>MSGGSTDVAMLSWLAALPATLGQVKDLEITSFKYDGQRGEVRIHARSSDFQPFEQARVKLAEKFNVEQGQLNRSDNVVMGSFVL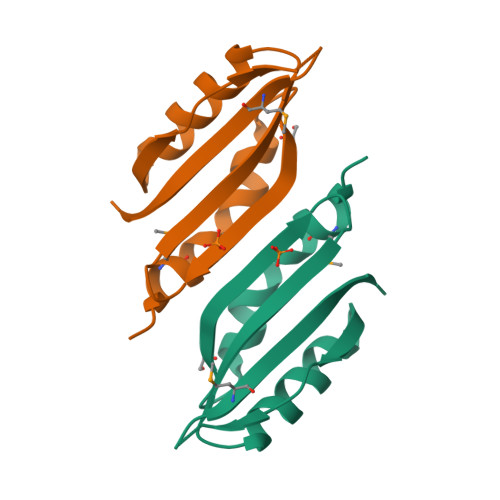KRQLEHHHHHH[2x]> GPLGSLTMGAQDTLPVAAAFTETVNAYFKGADPSKCIVKITGEMVLSFPAGITRHFANNPSPAAL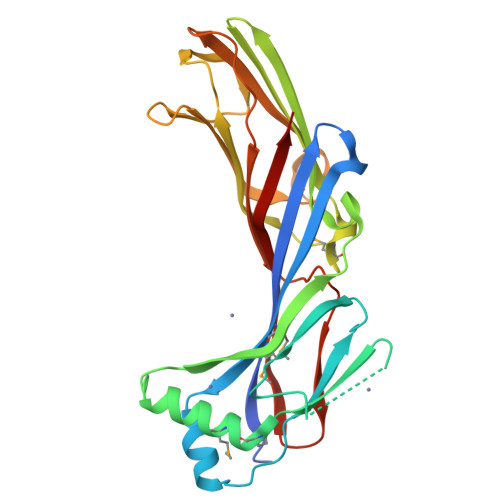TFRVINFSRLEHVLPNPQLLCCDNTQNDANTKEFWVNMPNLMTHLKKVSEQKPQATYYNVDMLKYQVSAQGIQSTPLNLAVNWRCEPSSTDLRIDYKYNTDAMTTAVALNNVQFLVPIDGGVTKLQAVLPPAVWNAEQQRILWKIPDISQKSENGGVGSLLARFQLSEGPSKPSPLVVQFTSEGSTLSGCDIELVGAGYRFSLIKKRFAAGKYLADN The BEN domain, which is named after the exemplar proteins BANP, E5R and NACC1 (also known as NAC1), is found in diverse animal and viral proteins and has been shown to constitute a new class of DNA-binding domain (DBD) (1–4). There are nine BEN domain-containing proteins in humans, including BANP, BEND2–7, NACC1 and NACC2. Over the past few years, studies have demonstrated the preferred DNA sequences for some human BEN domain proteins, which can be roughly classified into two groups based on their recognized motifs. In this study, we solved the crystal structures of DNA-bound BEN domains from both BANP and NACC1, which are representative members of each group of BEN domain proteins.

The first group of proteins includes NACC1 and NACC2, both of which recognize sequences containing a conserved CATG motif. To clarify the molecular basis of DNA recognition by NACC1, we solved the crystal structure of the BEN domain of NACC1 in complex with bound 10-bp CATG-containing DNA with a thymine overhang at the 5′ end at a resolution of 2.3 Å. In the structure, the BEN domain of NACC1 contains two β-strands at the N-terminus and five α-helices that fold into a globular structure. In this complex, one NACC1 molecule binds one double-stranded DNA molecule. Sequence-specific DNA recognition is mediated primarily by the C-terminal helix α5 of the NACC1 BEN domain, which inserts into the major groove and contacts the bases inside. Asp462 from α5 forms a hydrogen bond each with the bases of C4 and A5 from one chain of DNA. Thr465 and Arg469 from α5 recognize bases from the other chain of DNA, with Thr465 forming a hydrogen bond with A6′ and Arg469 forming a pair of hydrogen bonds with G4′, respectively. Notably, nearly half of the loop between α3 and α4 hangs over the neighbouring minor groove, with the long side chain of Arg421 from this loop inserting into the narrow minor groove and forming a pair of hydrogen bonds with the base of T10′. Overall, NACC1 covers a length of 10 bp on the DNA substrate. The insertion of the α5 helix widens the CATG-containing major groove by 1–2 Å.

>GSASLPAELINQIGNRCHPKLYDEGDPSEKLELVTGTNVYITRAQLMNCHVSAGTRHKVLLRRLLASFFDRNTLANSCGTGIRSSTNDPRRKPLDSRVLHAVKYYCQNFAPNFKESEMNAIAADMCTNARRVVRKSWMP[4x]>[8x]MALDAFSKVVTNADAKAAYVGGADLQALKKFISEGNKRLDAVNSIVSNASCIVSDAVSGMICENPSLISPSGNCYTNRRMAACLRDGEIILRYVSYALLSGDSSVLEDRCLNGLKETYSSLGVPANSNARAVSIMKACAVAFVNNTASQRKLSTPQGDCSALASEVAGYFDKVSAAIG;>AFDKSAKAPVITIFDHRGCTAHKNAEYKGALTNSIDDEMCVKVQSVKIAVSEADAAKKLQEFISYEAKGIDGAYTGRK[4x];>[4x]ADDKSGKAPVITVFDHRGCQRGGPDREYKGKKANGPDDEMCVKVQSAKIAVSATTADSVLQQTISTLYRK

In addition to their membrane‐bound chlorophyll a/c light‐harvesting antenna, the cryptophyte algae have evolved a unique phycobiliprotein antenna system located in the thylakoid lumen. The basic unit of this antenna consists of two copies of an αβ protomer where the α and β subunits scaffold different combinations of a limited number of linear tetrapyrrole chromophores. While the β subunit is highly conserved, encoded by a single plastid gene, the nuclear‐encoded α subunits have evolved diversified multigene families. By careful examination of three newly determined crystal structures in comparison with three previously obtained, we show how the α subunit amino acid sequences control chromophore conformations and hence spectral properties even when the chromophores are identical.

The crystal structure of PE566 has four copies of the closed form (αLβ).(αSβ) complex in the asymmetric unit. The structure of PE566 is most like that of PE545 (RMSD 0.23 Å over Cα 266 atoms), with near identity between the β subunits (167/178 residues) and significant identity in the α subunits (sequence identity: αL—48/78 residues; and αS—39/70 residues). In contrast to the two previous examples, the spectral difference between PE566 and PE545 is primarily due to different chromophores. In contrast, the α19 chromophore of PE566 is bilin 618 and two sites on the β subunit, β50/61 and β158, have bilin 584 chromophores, while the β82 chromophore is PEB, as per PE545 (Note: the PE566 β subunit has an additional residue at the N‐terminus, hence the bilins are actually attached to Cys51, Cys62, Cys83, and Cys159, however, we keep the conventional bilin nomenclature to facilitate comparison between proteins). We note that the presence of a double bond between the two central carbon atoms in the propionate side chains of pyrrole ring C in bilin 618 and bilin 584 is the only chemical feature that distinguishes these chromophores from DBV and PEB, respectively. Comparing the structures of PE566 and PE545 shows only a few distinguishing features. One notable difference is in the loop between helices hG and hH which differs in the β subunit attached to αL in the two structures. This loop interacts with pyrrole ring D in the β50/61 chromophore of its neighboring β subunit with the aliphatic portion of Lys151 making van der Waals contact with the face of pyrrole ring D. In contrast, this surface is solvent exposed in PE545. Despite having no sequence similarity and being one residue longer, the structure of the chromophore loop (residues Thr19 to Ile34) in PE566 αL is nearly identical to that of PE545 with PE566 His22 and Glu26 forming a salt bridge that supports the central pyrrole rings of the α19 chromophore (vs. Arg21 and Glu25 in PE545) and the side chain of Glu26 making a hydrogen bond to the nitrogen in pyrrole ring D, as seen in PE545.>NKMVEYLTDWVMGTSNQAADDDVKCLTRDLDQASMEAVVSLLAGLPLQPEEGDGVELMEAKSQLFLKYFTLFMNLLNDCSEVEDESAQTGGRKRGMSRRLASLRHCTVLAMSNLLNANVDSGLMHSIGLGYHKDLQTRATFMEVLTKILQQGTEFDTLAETVLADRFERLVELVTMMGDQGELPIAMALANVVPCSQWDELARVLVTLFDSRHLLYQLLWNMFSKEVELADSMQTLFRGNSLASKIMTFCFKVYGATYLQKLLDPLLRIVITSSDWQHVSFEVDPTRLEPSESLEENQRNLLQMTEKFFHAIISSSSEFPPQLRSVCHCLYQATCHSLLNKATVKEKKENKKSVVSQRFPQNSIGAVGSAMFLRFINPAIVSPYEAGILDKKPPPRIERGLKLMSKILQSIANHVLFTKEEHMRPFNDFVKSNFDAARRFFLDIASDCPTSDAVNHSLSFISDGNVLALHRLLWNNQEKIGQYLSSNRDHKAVGRRPFDKMATLLAYLGPPEHKPVADTHWSSLNLTSSKFEEFMTRHQVHEKEEFKALKTLSIFYQAGTSKAGNPIFYYVARRFKTGQINGDLLIYHVLLTLKPYYAKPYEIVVDLTHTGPSNRFKTDFLSKWFVVFPGFAYDNVSAVYIYNCNSWVREYTKYHERLLTGLKGSKRLVFIDCPGKLAEHIEHEQQKLPAATLALEEDLKVFHNALKLAHKDTKVSIKVGSTAVQVTSAERTKVLGQSVFLNDIYYASEIEEICLVDENQFTLTIANQGTPLTFMHQECEAIVQSIIHIRTRWELSQPDSIPQHTKIRPKDVPGTLLNIALLNLGSSDPSLRSAAYNLLCALTCTFNLKIEGQLLETSGLCIPANNTLFIVSISKTLAANEPHLTLEFLEECISGFSKSSIELKHLCLEYMTPWLSNLVRFCKHNDDAKRQRVTAILDKLITMTINEKQMYPSIQAKIWGSLGQITDLLDVVLDSFIKTSATGGLGSIKAEVMADTAVALASGNVKLVSSKVIGRMCKIIDKTCLSPTPTLEQHLMWDDIAILARYMLMLSFNNSLDVAAHLPYLFHVVTFLVATGPLSLRASTHGLVINIIHSLCTCSQLHFSEETKQVLRLSLTEFSLPKFYLLFGISKVKSAAVIAFR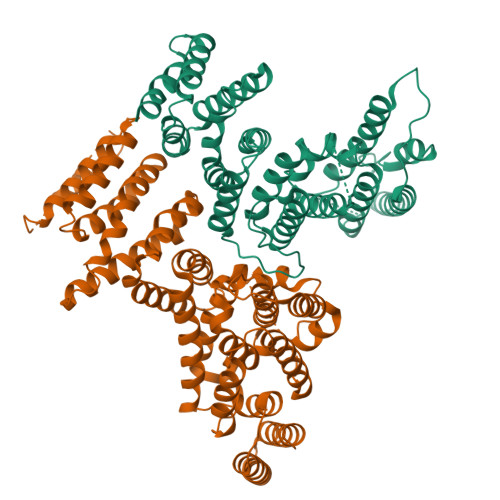SSYRDRSFSPGSYERETFALTSLETVTEALLEIMEACMRDIPTCKWLDQWTELAQRFAFQYNPSLQPRALVVFGCISKRVSHGQIKQIIRILSKALESCLKGPDTYNSQVLIEATVIALTKLQ[2x]(2S)-2-phenylpropane-1-sulfonamide | C9 H13 N O2 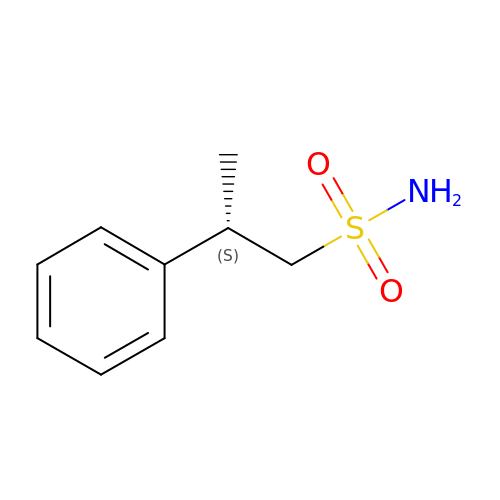S | HXLOQIXEAPZOSG-MRVPVSSYSA-N>[2x]HHHHHHGSERTGTQPLGVQGLTEEQRMMIRELMDAQMKTFDTTFSHFKNFRLPGV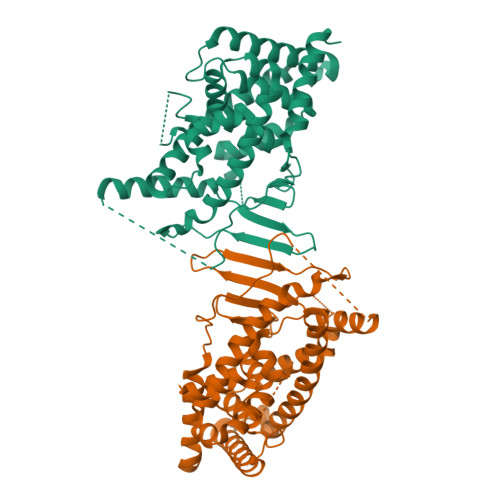LSSGCELPESLQAPSREEAAKWSQVRKDLCSLKVSLQLRGEDGSVWNYKPPADSGGKEIFSLLPHMADMSTYMFKGIISFAKVISYFRDLPIEDQISLLKGAAFELCQLRFNTVFNAETGTWECGRLSYCLEDTAGGFQQLLLEPMLKFHYMLKKLQLHEEEYVLMQAISLFSPDRPGVLQHRVVDQLQEQFAITLKSYIECNRPQPAHRFLFLKIMAMLTELRSINAQHTQRLLRIQDIHPFATPLMQELFGITGSSGGSGGSSHSSLTERHKILHRLLQEGSPSDITTLSVEPD> EKRLT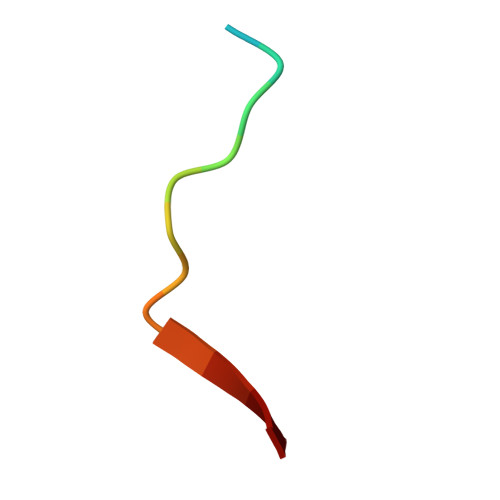LPPSEITLL2-HYDROXYMETHYL-5-(7-METHYLAMINO-3H-PYRAZOLO[4,3-D]PYRIMIDIN-3-YL)-TETRAHYDRO-FURAN-3,4-DIOL 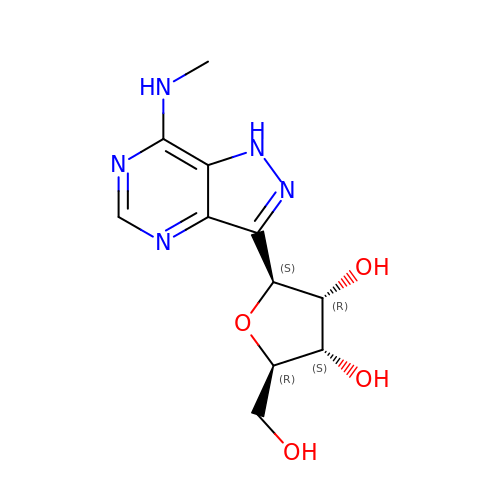| C11 H15 N5 O4 | JRRNRCMIBCSOIH-LFAOKBQASA-N> EFDVSTSELNQFDFWVQYAAAA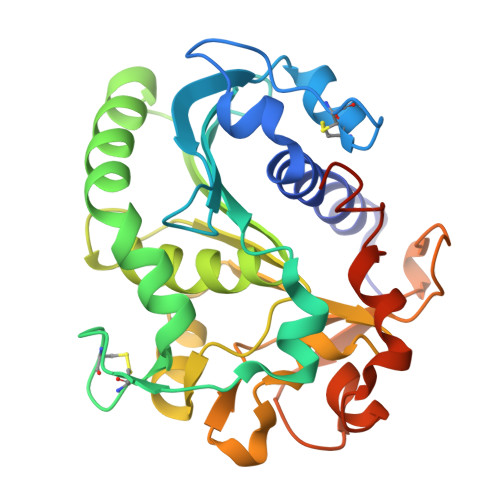YYADDYTAQVGAKISCSKGNCPQVEEAGATVFYDFSNATITDTSGFIAVDHANEAVVLSFRGSYSVRNWVSDAIFVYTNPDLCDGCLADLGFWGSWVLVRDDIIKELKEAVSQNPGYELAVVGHSLGAAVATLAVADLRGKGYPSAKLYAYASPRVANVPLAKHITAQGNNYRFTHTDDPVPKLPLLAMGYVHISPEYWITSPNNVTVGASDIKVIDGDISFAGNTGTGLPSLEDFEAHKWYFMKTDAGKNDGRPFKRVVD> MGSDKIHHHHHHMIIQRVVLNSRPGKNGNPVAENFRVEEFSLLDALNEGQVQVRTLYLSVDPYMRCKMNEDTGTDYLAPWQLAQVADGGGIGIVEESKHQKLAKGDFVTSFYWPWQTKAILDGNGLEKVDPQLVDGHLSYFLGAIGMPGLTSLIGVQEKGHISAGSNQTMV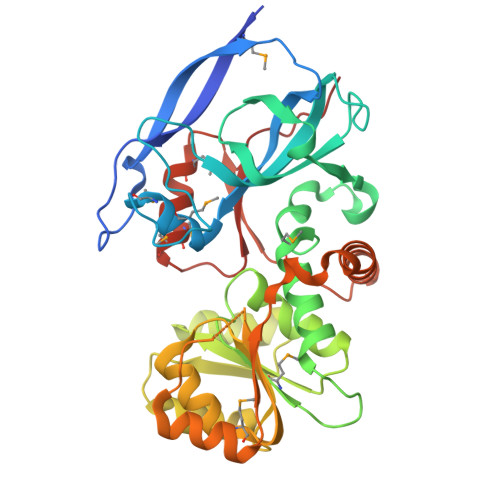VSGAAGACGSLAGQIGHLLGCSRVVGICGTQEKCLFLTSELGFDAAVNYKTGNVAEQLREACPGGVDVYFDNVGGDISNTVISQMNENSHIILCGQISQYNKDVPYPPPLPPAVEAIRKERNITRERFTVLNYKDKFEPGILQLSQWFKEGKLKVKETVAKGLENMGVAFQSMMTGGNVGKQIVCISEDSSL> MSAPPNTLFLRLEGALQSWGSNEAKFALRRTADAPTKSGVLGLLCAAMGIGRAEAADSWLPKLANLRMGVRIDRPGIRWWDFHTVGAGQRMRMAELKAPKKPSMVGAALAETLTPSKVKTRAETLLSRREYLADASFLVALQGEPELVAKLSAALAKPVWAIYLGRKSCPPSRPVCEHPPGFYNTLEEALSAVPLQKRWHNEPLPQILPCVMDWIPGYDGEHAPDDAEIHYDLPVSFQPPRHLPRFVIRRELVVGEDVQVSRETGTSVWRPKGTRADYNNSEYKKVRAERLVMDHAACMVCKHPATTVQHVNYRRAGGKEIPEDLRALCRLCHDACTMLEYGSGMTTNRIDPCDPIWRERILAKRKEIVEFRSRGQRFRKMKPEEENG;>MLIEIHMIQNHSPANLNRDDLGAPKTCYFGGVLRSRISSQCIKRSIRTSNDFKALLGGVRTRRLADLIQQEAGETECWKKAQEILNKCGFKNKDDNTKMLVFMSKDKIKDLARIVLDNSLGLTEAAQQVANVIAQATLAPDIALCGRMLE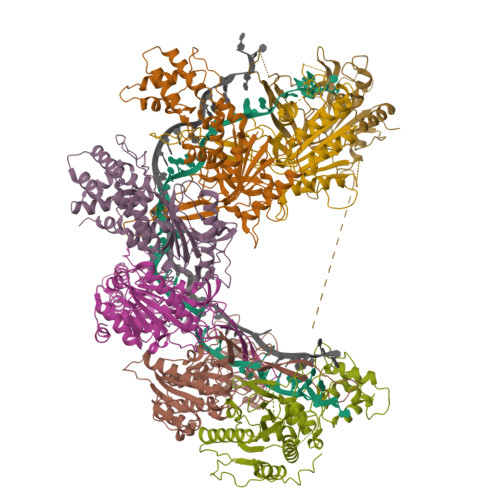PNDKDKDKKVKWSNTTVEAALQVAHAISTHIARPEIDYFVAADDVPGEDAGAGHIGESMFASACFYKYFSIDWEQLVKNLKGDTNLAAHTVGAFLLAAAKTNPSGKQNSFAAHNYPDGILVEFKNSPISYANAFVRPVSVVKESDLVEQSIGQLSNYVNDIRLGYYDEQSPVIGFWFSPNNRYPLGYKHSKLASRNIGNLNELVGAVLDYIGGFKWEEVQKSKAYIGG[6x]> HHHHHHAPAFRYTRSQSFDIFDINQKCFVLESPTQLVALHLQGPSSSQKVRLNIALYRPRGPRGSAGTGQMPVALGIKGYKLYMSCVMSGTEPTLQLEEADVMRDIDS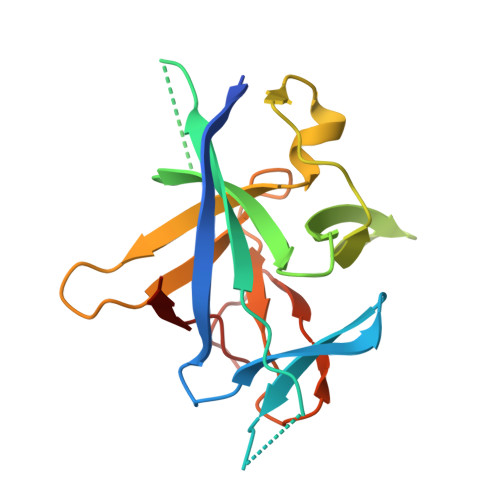VELTRFIFYRLDSPTAGTTRFESAAFPGWFICTSLQPRQPVGITNQPDQVNIATYKLSGR> GRLAGLSAALLRTDSFVGGRWLPAAATFPVQDPASGAALGMVADCGVREARAAVRAAYEAFCRWREVSAKERSSLLRKWYNLMIQNKDDLARIITAESGKPLKEAHGEILYSAFFLEWFSEEARRVYGDIIHTPAKDRRALVLKQPIGVAAVITPWNFPSAMITRKVGAALAAGCTVVVKPAEDTPFSALALAELASQAGIPSGVYNVIPCSRKNAKEVGEAICTDPLVSKISFTGSTTTGKILLHHAANSVKRVSMELGGLAPFIVFDSANVDQAVAGAMASKFRNTGQTAVCSNQFLVQRGIHDAFVKAFAEAMKKNLRVGNGFEEGTTQGPLINEKAVEKVEKQVNDAVSKGATVVTGGKRHQLGKNFFEPTLLCNVTQDMLCTHEETFGPLAPVIKFDTEEEAIAIANAADVGLA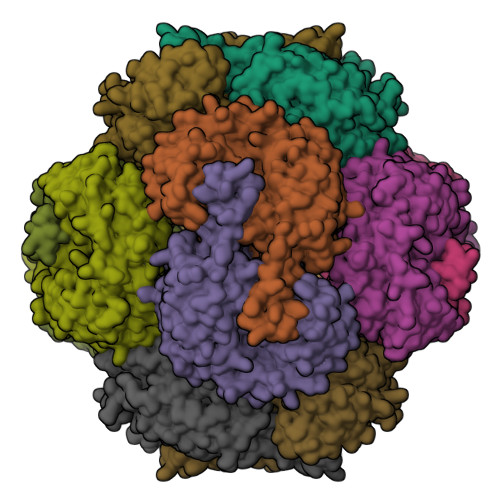GYFYSQDPAQIWRVAEQLEVGMVGVNEGLISSVECPFGGVKQSGLGREGSKYGIDEYLELKYVCYGGL>[2x]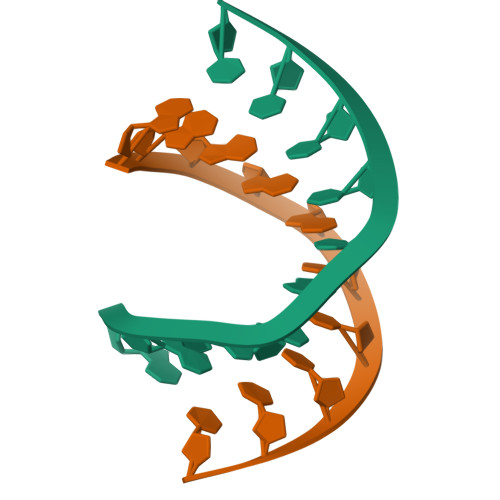AGGGGCCCCT> DSISLSLINEGPSYASKVSVGSNKQQQTVIIDTGSSDFWVVDSNAQCGKGVDCKSSGTFTPSSSSSYKNLGAAFTIRYGDGSTSQGT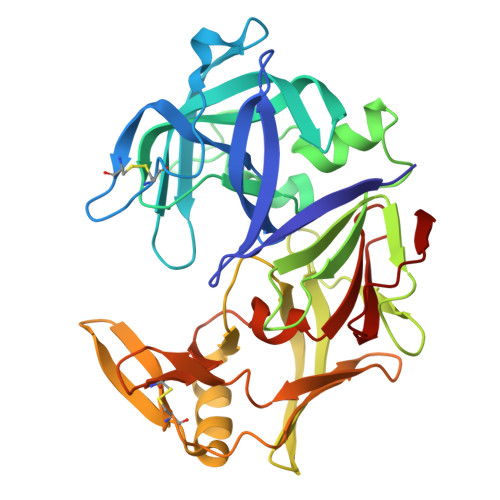WGKDTVTINGVSITGQQIADVTQTSVDQGILGIGYTSNEAVYDTSGRQTTPNYDNVPVTLKKQGKIRTNAYSLYLNSPSAETGTIIFGGVDNAKYSGKLVAEQVTSSQALTISLASVNLKGSSFSFGDGALLDSGTTLTYFPSDFAAQLADKAGARLVQVARDQYLYFIDCNTDTSGTTVFNFGNGAKITVPNTEYVYQNGDGTCLWGIQPSDDTILGDNFLRHAYLLYNLDANTISIAQVKYTTDSSISAV>[2x]MRSRRVDVMDVMNRL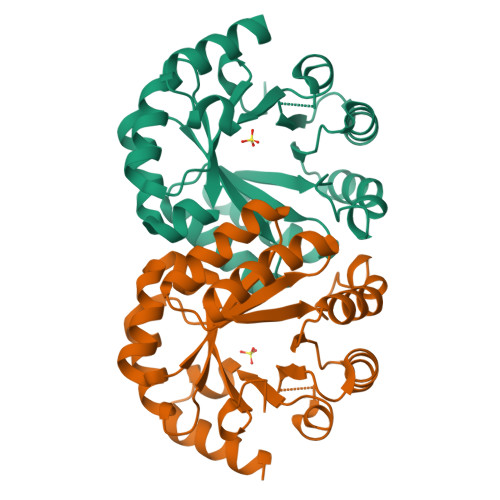ILAMDLMNRDDALRVTGEVREYIDTVKIGYPLVLSEGMDIIAEFRKRFGCRIIADFKVADIPETNEKICRATFKAGADAIIVHGFPGADSVRACLNVAEEMGREVFLLTEMSHPGAEMFIQGAADEIARMGVDLGVKNYVGPSTRPERLSRLREIIGQDSFLISPGAGAQGGDPGETLRFADAIIVGRSIYLADNPAAAAAGAIESIKDLLNP> MSDQEAKPSTEDLGDKK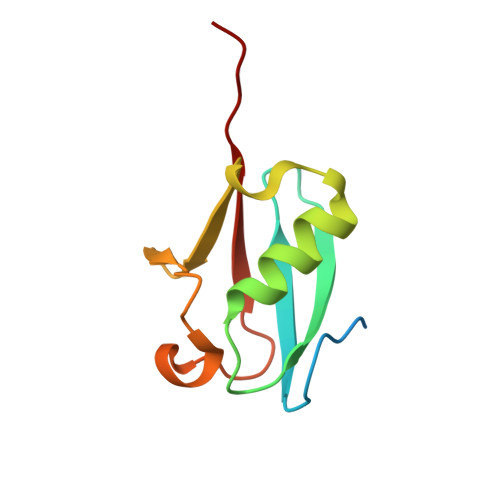EGEYIKLKVIGQDSSEIHFKVKMTTHLKKLKESYCQRQGVPMNSLRFLFEGQRIADNHTPKELGMEEEDVIEVYQEQTGG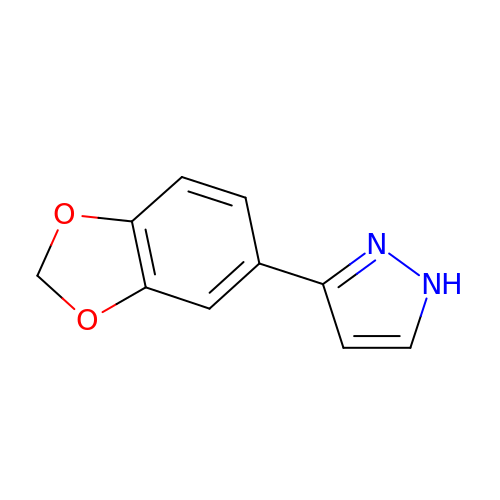(3P)-3-(2H-1,3-benzodioxol-5-yl)-1H-pyrazole | C10 H8 N2 O2 | LOPAFWMOCZGHFX-UHFFFAOYSA-N Thus, the BBSome is a key regulator of the composition of transmembrane proteins in the ciliary membrane, and is thought to be evolutionarily related to other transmembrane protein trafficking complexes including clathrin coats and the COPI and COPII coatomers. The recruitment of the BBSome to ciliary membranes (where it binds transmembrane protein substrates) is mediated by a highly specific interaction with ARL6 (also known as BBS3). Here, we use single-particle cryo-EM to determine structures of the native bovine BBSome complex with and without ARL6 at 3.5 Å and 3.1 Å resolution, respectively. The structures reveal the mechanism of ARL6-mediated activation and provide new insights into the pathogenesis of BBS-causing mutations and the evolutionary relationship between the BBSome and other transmembrane protein trafficking complexes.

However, our 3.5 Å resolution structure of the BBSome:ARL6:GTP complex shows that the head remains in a closed, downward conformation even in the presence of ARL6. Rather, BBS1βprop swivels in its cradle between BBS4 and BBS7 to accommodate ARL6. This swiveling action involves a rotation of approximately 25° and a movement of 13 Å away from BBS2βprop. The N-terminal half of BBS4 shows a small 2–3 Å displacement to accommodate the movement of BBS1βprop. The swiveling of BBS1βprop opens a central cavity in the BBSome with dimensions of 50 × 15 Å, wide enough to accommodate a polypeptide chain. This cavity is flanked by the newly exposed edges of BBS1βprop, BBS2β-prop and BBS7βprop as well as BBS4 and BBS8 in the body. The first and last blades of BBS1βprop interact with the switch two loop and helices α3 (residues 75–78) and α4 (residues 98–108) of the GTP-bound ARL6. Density for GTP and the ordered switch loops of ARL6 are clearly visible in our reconstruction. We also see an additional interaction between ARL6 and the loop that connects BBS7βprop with BBS7hx (residues 320–335). This linker is disordered in the BBSome-only structure but binds along the β-edge of the central β-sheet of ARL6.

> MAETKSMFREVLPKQGQLYVEDITTMVLCKPKLLPLKSLTLEKLEKMQQAAQDTIHQQEMTEKEQKITH;> MAATSSSDSDGGKGESEANSKWLDSLSDSMANIHTFSACLALADFHGDGEYKLAMGDLGPDGRQPRLKVLKGHTLVSQKPLPDLPAAAVTFLMASHEPRTPALAIASGPCVYVYKNLKPYFKFSLPSLPTNPLEQDLWNQAKEDQIDPLTLKEMLEGIREKAEVPLSVQSLRFLPLELSEMEAFVNQHKSKSIRRQTVITTMTTLKKNLADEDAVSCLVLGTENKELLVLDPEAFTILAKMSLPSVPAFLEASGQFDVEFRLAAACRNGSIYILRRDSKRPKYCIELGAQPVGLVGVHKVLVVGSNQDSLHGFTYKGKRLWTVQMPAAILAMNLLEQHSRGLQAVMAALANEEVRIYHDKVLLNVIRTPEAVTSLCFGRYGREDNTLIMTTLGGGLIIKILKRTAVFAEGGGEAGPPPSQAIKLNVPRKTRLYVDQTLREREAGTAMHRTFQADLYLLRLRAARAYVQALESSLSPVSLTAREPLKLHAVVQGLGPTFKLTLHLQNTSTARPILGLVVCFLYNEVLYALPRAFFKVPLLVPGLNYPLETFVKSLSDKGISDIIKVLVLREGQSTPLLSAHINMPMSEGLAAD;> MLQPVFTLKLRHKISPRMVAVGRYDGTHPCLAAATQAGKVFIHNPHSRSQHLGAPRVLQSPLESDVSLLNINQTVSCLTAGVLNPELGYDALLVGTQTNLLAYDVYNNSDLFYREVADGASAIVLGTLGDITSPLAIIGGNCALQGFNHEGNDLFWTVTGDNVHSLALCDFDGDGKKELLVGSEDFDIRVFKEDEIVAEMSETEIITSLCPMYGSRFGYALSNGTVGVYDKTARYWRIKSKNQAMSIHAFDLNSDGVCELITGWSNGKVDARSDRTGEVIFKDNFSSAIAGVVEGDYRMEGCQQLICCSVDGEIRGYLPGTAEMRGNLMDISVEQDLIRELSQKKQNLLLELRNYEENAKAELSSPLNEADGHRGVIPANTKHHTALSVSLGSEAQAAHAELCISTSNDTIIRAVLIFAEGVFAGESHVVHPSVHHLSSSVRIPITPPKDIPVDLHLKTFVGYRSSTQFHVFELTRQLPRFSMYALTSPDPASEPLSYVNFIIAERAQRVVMWLNQNFLLPEDTNIQNAPFQVCFTSLRNGGQLYIKIKLSGEITVNTDDIDLAGDIIQSMASFFAIEDLQVEADFPVYFEELRKVLVKVDEYHSVHQKLSADMADNSNLIRSLLVQAEDARLMRDMKTMKNRYKELYDLNKDLLNGYKIRCNNHTELLGSLKAVNQAIQRAGHLRVGKPKNQVITACRDAIRSNNINMLFRIMRVGTASS;> MGLLDRLSGLLGLKKKEVHVLCLGLDNSGKTTIINKLKPSNAQSQDIVPTIGFSIQKFKSSSLSFTVFDMSGQGRYRNLWEHYYKEGQAIIFVIDSSDKLRMVVAKEELRTLLNHPDIKHRRIPILFFANKMDLRDALTSVKVSQLLCLEDIKDKPWHICASDAIKGEGLQEGVDWLQDQIQSVKT;> MAEEKLSARTQLPVSAESQKPVLKKAPEFPILEKQNWLIHLYYIQKDYEACKAVIKEQLQETHGLCEYAIYVQALIFRLEGNIQESLRLFQMCAFLSPQCADNLKQVARSLFLLGKHKAAIEVYNEAAKLNQKDWEICHNLGVCYIYLKQFDKAQDQLHNALHLNRHDLTYIMLGKIFLLKGDLDKAIEIYKKAVEFSPENTELLTTLGLLYLQLGIYQKAFEHLGNTLTYDPTNYKAILAAGSMMQTHGDFDVALTKYKVVACAVIESPPLWNNIGMCFFGKKKYVAAISCLKRANYLAPLDWKILYNLGLVHLTMQQYASAFHFLSAAINFQPKMGELYMLLAVALTNLEDSENAKRAYEEAVRLDKCNPLVNLNYAVLLYNQGEKRDALAQYQEMEKKVNLLKYSSSLEFDPEMVEVAQKLGAALQVGEALVWTKPVKDPKSKHQTASTSKAAGFQQPLGSNQALGQAMSSAATCRKLSSGAGGTSQLTKPPSLPLEPEPTVEAQPTEASAQTREK;> MSVLDALWEDRDVRFDVSSQQMKTRPGEVLIDCLDSVEDTKGNNGDRGRLLVTNLRIVWHSLALPRVNLSIGYNCILNITTRTANSKLRGQTEALYVLTKCNSTRFEFIFTNLVPGSPRLYTSLIAVHRAYETSKMYRDFKLRSALIQNKQLRLLPQENVYNKINGVWNLSSDQGNLGTFFITNVRIVWHANMNDSFNVSIPYLQIRSVKIRDSKFGLALVIESSQQSGGYVLGFKIDPVEKLQESVKEINSLHKVYSANPIFGVDYEMEEKPQPLEALTVKQIQDDVEIDSDDHTDAFVAYFADGNKQQDREPVFSEELGLAIEKLKDGFTLQGLWEVMN;> MDLNLNRADYLQVGVTSQKTMKLLPASKHRATQKVVVGDHDGIVMCFGMKKGEAVTVFKTLPGQKIARLELGGALNTPQEKIFIAAGSEIRGFTKRGKQFLSFETNLTESIKAMHISGSDLFLSASYIYNHYCDCKDQHYYLSGDKINDVICLPVERLLREVPVLACQDRVLRVLQGSDVTYEIEVPGPPTVLALHNGNGGDSGEDLLFGTSDGKLGLIQITTSKPIHKWEIRNEKKRGGILCVDSFDIVGDGVKDLLVGRDDGMVEVYGFDNANEPVLRFDHTLSESVTSIQGGCVGKDGYDEIVVSTYSGWITGLTTEPVHKESGPGEELKFNQEMQNKISSLRSELEQLQYKVLQEREKYQQSSQSSKAKSAVPSFSVNDKFTLNKDDASYSLILEVQTAIDNVLIQSDVPIDLLDVDKNSAVVSFSSCDSESNDNFLLATYRCQANTTRLELKIRSIEGQYGTLQAYVTPRIQPKTCQVRQYHIKPLSLHQRTHFIDHDRPMNTLTLTGQFSFSELHSWVVFCMPEVPEKPPAGECVTFYFQNTFLDTQLESTYRKGEGVFKSDNISTISILKDVLSKEATKRKINLNISYEINEVSVKHTLKLIHPKLEYQLLLAKKVQLIDALKELQVHEGNTNFLIPEYRCILEEADHLQEEYKKQPAHLERLYGMITDLFIDKFKFKGTNVKTKVPLLLEILDSYDQNALIAFFDAA;> MEPLLLAWSYFRRRRFQLCADLCTQMLEKSPCDQAAWILKARALTEMVYVDEIDVDEEGIAEMILDENAIAQVPRPGTSLKLPGTNQTGGPSPAVRPVTQAGRPITGFLRPSTQSGRPGTIEQAIKTPRTAYTARPIASSSGRFVRLGTASMLTSPDGPFINLSRLNLAKYAQKPKLAKALFEYIFHHENDVKTALDLAALSTEHSQYKDWWWKVQIGKCYYRLGLYREAEKQFKSALKQQEMVDTFLYLAKVYISLDQPLTALNLFKQGLDKFPGEVTLLCGIARIYEEMNNISSATEYYKEVLKQDNTHVEAIACIGSNHFYTDQPEVALRFYRRLLQMGVYNCQLFNNLGLCCFYAQQYDMTLTSFERALSLAENEEEVADVWYNLGHVAVGTGDTNLAHQCFRLALVSNNQHAEAYNNLAVLEMRRGHVEQAKALLQTASSLAPHMYEPHFNFATISDKIGDLQRSYAAAKKSEAAFPDHVDTQHLIKQLEQHFAML;> MSLFKARDWWSTVLGDKEEFDQGCLCLADVDNTGNGQDKIIVGSFMGYLRIFNPHPVKTGDGAQAEDLLLEVHLRDPILQVEVGKFVSGTEMLHLAVLHSRKLCVYSVSGTLGNVEHGNQYQIKLMYEHNLQRTACNMTYGSFGGVKGRDLICIQSVDGMLMVFEQESYAFGRFLPGSLLPGPLAYSSRTDSFITVSSCHQVESYKYQVLAFATDADKRQETEQQKHGSGKRLVVDWTLNIGEQAIDICIVSFIQSASSVFVLGERNFFCLKDNGQIQFMKKLDYSPSCFLPYCSVSEGTINTLIGNHNNMLHIYQDVTLKWATQLPHVPVAVRVGCLHDLKGVIVTLSDDGHLQCSYLGTDPSLFQAPKVESRELNYDELDMELKELQKVIKNVNKSQDVWPLTEREDDLKVSAMVSPNFDSVSQATDVEVGADLVPSVTVKVTLKNRVALQKIKLSIYVQPPLVLTGDQFTFEFMAPEMTRTVGFSVYLKGSYSPPELEGNAVVSYSRPTERNPDGIPRVSQCKFRLPLKLVCLPGQPSKTASHKLTIDTNKSPVSLLSLFPGFAKQSEDDQVNVMGFRFLGGSQVTLLASKTSQRYRIQSEQFEDLWLITNELIIRLQEYFEKQGIKDFTCSFSGSVPLEEYFELIDHHFELRINGEKLEELLSERAVQFRAIQRRLLTRFKDKTPAPLQHLDTLLDGTYKQVIALADAVEENQDNLFQSFTRLKSATHLVILLIGLWQKLSADQIAILEAAFLPLQQDTQELGWEETVDAALSHLLKTCLSKSSKEQALNLNSQLGIPKDTSQLKKHITLFCDRLAKGGRLCLSTDAAAPQTMVMPGGCATIPESDLEGRSIDQDSSELFTNHKHLMVETPVPEVSPLQGVTE>[4x]SNASGQQVHRLLGNKLELASTGQTIYHQDINLNNHPWIGDHRVYDTPVIPGVSYIAMTLAAVGVPAAVEDINFQQPLFLAESNTTRETQLMLHTADNVGKQFVEVFSRDGAKQEEWQQHASMSVSENPPPPPTLSVDIPALCEQLRPLDTDTLTEIYASISLVYGPMLQAVRQAWIGEETSLLEIEVPKALAFQLAGEPIHPVLI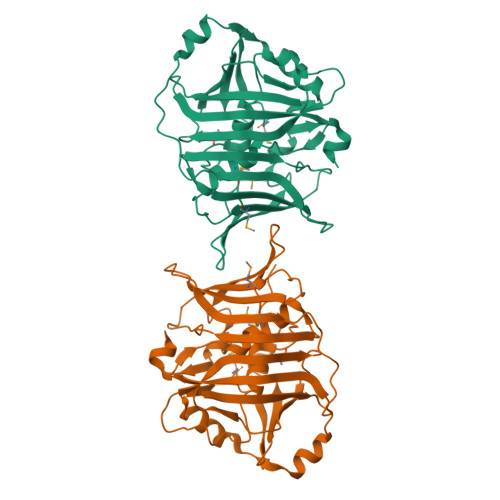DACTRLTPDLFDFSSDSGVFWAPWRVKEMTLSHPTPSRFYAYVEEPSRVNEQLQTRSYDIQLLDETGQAFGRINGFTVKRAPSQLFLK> ADTYAATRYPVILVHGLAGTDKFANVVDYWYGIQSDLQSH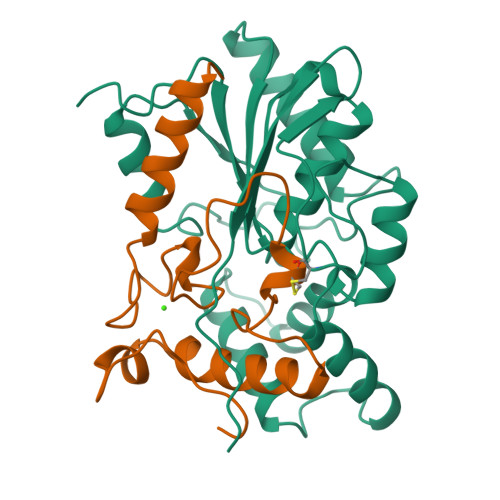GAKVYVANLSGFQSDDGPNGRGEQLLAYVKQVLAATGATKVNLIGHSQGGLTSRYVAAVAPQLVASVTTIGTPHRGSEFADFVQDVLKTDPTGLSSTVIAAFVNVFGTLVSSSHNTDQDALAALRTLTTAQTATYNRNFPSAGLGAPGSCQTGAATETVGGSQHLLYSWGGTAIQPTSTVLG;> VVGATDTSTGTLDVANVTDPSTLALLATGAVMINRASGQNDGLVSRCSSLFGQVISTSYHWNHLDEINQLLGVRGANAEDPVAVIRTHVNRLKLQGV> KTYRRSYTHAKPPYSYISLITMAIQQSPNKMLTLSEIYQWIMDLFPFYRQNQQRWQNSIRHSLSFNDCFLKVPRSPDKPGKGSFWTLHPDSGNMFENGCYLRRQKRFKCEKQLALKEAAGAAGSG

Forkhead box H1 (FoxH1) is an essential maternal pioneer factor during embryonic development that binds to specific GG/GT-containing DNA target sequences. The members of the FOX transcription factor family share the presence of the forkhead domain (FH), which interacts with DNA (InterPro entry IPR001766). Most FOX proteins recognize the canonical forkhead DNA motif TRTTTRY (R = A/G, Y = C/T). In contrast, FoxH1 recognizes the TGTG(G/T)ATT sequences in several cis-regulatory elements, such as in Gsc, Eomes, Nodal, Mixl, and FoxA2, to confer activin regulation in vivo.

In contrast, FoxA2, also a pioneer factor that binds to canonical forkhead motifs, displayed the opposite behavior and selected only for DNAs with TT sites, even showing a decrease in its melting temperature in the presence of the GG site. Also, EMSA assays indicated that FoxA2 binds weakly to the TGTGGATT site whereas it interacts with high affinity with its forkhead site. To explore the impact of the protein-DNA interactions on the DNA topology, we compared the DNA shapes of the FoxH1 complexes with other FOX structures available in the PDB and with the pair of complexes we determined here for FoxA2 using Curves+ 43. Small differences were detected at the major groove, whereas the minor grooves were found to be slightly wider in the FoxH1 complexes than in other FOX structures. A similar absence of interaction between Asn and the G-C pair could account for the DNA binding preferences of FoxA2. The structural information we gathered for the DNA binding specificities of FoxA2 and FoxH1 FH domains is compatible with the hypothesis whereby FoxA proteins substitutes for FoxH1 preferentially at TT sites, with FoxH1 remaining bound to GK sites even when the concentration of this protein is low.>MGSSHHHHHHSQDPSQFIRRDIAQTVNGSLTLTQQTNLSAPLVSSSTGEFGGSLAANRTFTIRNTGAPTSIVFEKGPASGANPAQSMSIRVWGNQFGGGSDTTRSTVFEVGDDTSHHFYSQRNKDGNIAFNINGTVMPININASGLMNVNGTATFGRSVTANGEFISKSANAFRAINGDYGFFIRNDASNTYFLLTAAGDQTGGFNGLRPLLINNQSGQITIGEGLIIAKGVTINSGGLTVNSRIRSQGTKTSDLYTRAPTSDTVGFWSIDINDSATYNQFPGYFKMVEKTNEVTGLPYL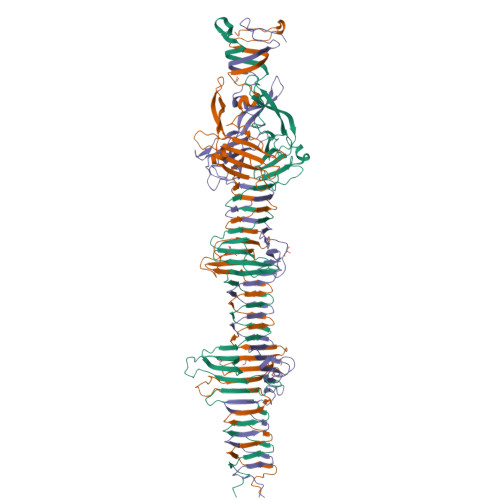ERGEEVKSPGTLTQFGNTLDSLYQDWITYPTTPEARTTRWTRTWQKTKNSWSSFVQVFDGGNPPQPSDIGALPSDNATMGNLTIRDFLRIGNVRIVPDPVNKTVKFEWVE[3x]> MHHHHHHGGGGGMYDVVILAGGLGTRLKSVSGDIPKPMVDISGKPFLYRLMEYLEDQGVQRIILSLSYKADYIIDSLIKDNPVNSKVDFIIENEPLGTGGAIKNACKYIEASKFIVINGDTYCELDYKKFIESSLDSDLQISGVEVDDVCR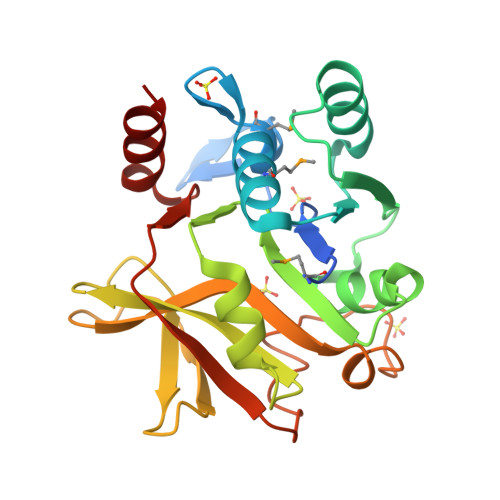YGSLDIDHDFHVNSIVEKGHQGTGIINSGTYILSKKIIEDYPHDKFSFELDFLPKFTGVFKAFVTKAYFIDIGIPEDYYKACEKFK>EFGTFLNLTKPLCEVSSWHILSKDNAIRIGEDAHILVTREPYLSCDPQGCRMFALSQGTTLRGRHANGTIHDRSPFRALISWEMGQAPSPYNVRVECIGWSSTSCHDGISRMSICMSGPNNNASAVVWYGGRPVTEIPSWAGNILRTQESECVCHKGICPVVMTDGPANNRAATKIIYFKEGK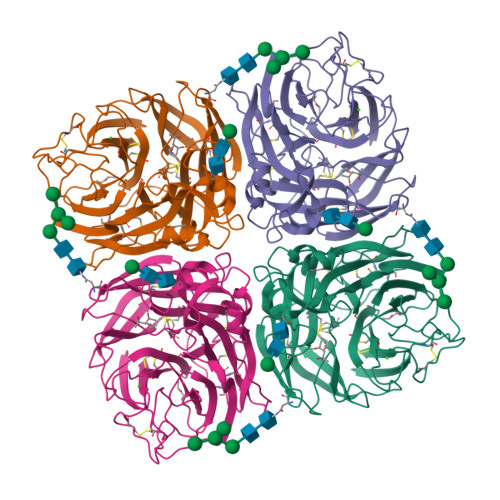IQKIEELAGNAQHIEECSCYGAVGVIKCVCRDNWKGANRPVITIDPEMMTHTSKYLCSKILTDTSRPNDPTNGNCDAPITGGSPDPGVKGFAFLDGENSWLGRTISKDSRSGYEMLKVPNAETDTQSGPISHQVIVNNQNWSGYSGAFIDYWANKECFNPCFYVELIRGRPKESSVLWTSNSIVALCGSKERLGSWSWHDGAEIIYFK[2x]> GASGSGTGSGSMLYLIIYDVPATKAGNKRRTRLFDLLSGYGKWRQFSVFECFLSVKQFAKLQTAMEKLIKLDEDA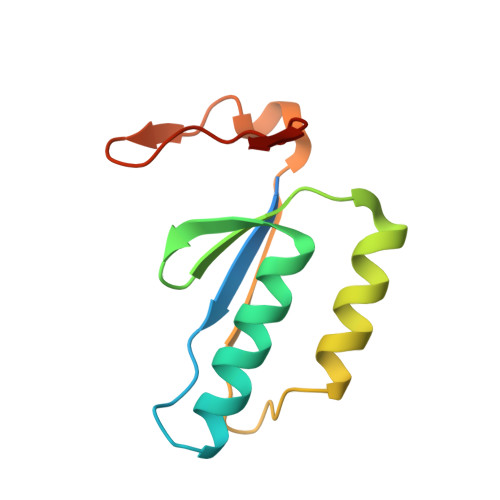VCIYVLDENTVQRTITYGTPQPEKPGSIII>GPGSIKPHKFWNTQPVVQNDDSSSEYSFGPIEIEPDSFRKEIYKLPDGFSWFDCNLWDIESQDFEDTYQLLKDHYVEDDDSQFRFNYSKEFLRWALCVPGQKKNWLVGVRVNETKKMVGFISAIPIKVRIHNCIMNTSVVNFLCVHKKLRSKRLAPVLIKEITRRIRCEKIFQSIYTCGKNITKPFTIGTYWHRIINVKKLLEAGFIGIPRNMTMSSLIKYHRIPADKRIEGFRPSVDSDAEQICKLFENYFMKYKDVSNETMNNLINY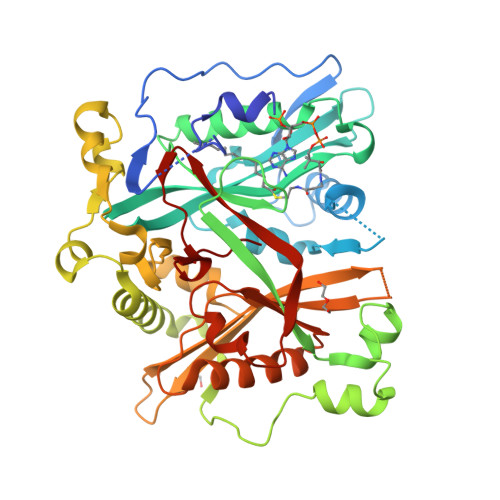DEINHSAALGKQAYMKLDKIEDLQDKITIHQCFNVEDVKHYFTNIDKVIVTYVRENKNKEITDLFSFFIIESTVINNERFPTINIAYSYFNIANTCSLKELFNEMLITAKNNNCDAFNTLDLMQNLQVIQDSKFIIGTGRLRYYVFNWKIPQISPSNVGIILF[2x]>GSHMIRIDATPYPYQFHPRSTALVVIDMQRDFIEEGGFGSALGNDVRPLAAIVPTVAALLQLAREAGMLVVHTRESHLPDLSDCPRSKRLRGNPTLGIGDVGPMGRILVQGEPGNQILPQLAPVEGELVIDKPGKGAFYATDLHAQLQERRITHLLVAGVTTEVCVQTSMREANDRGYECLVIEDA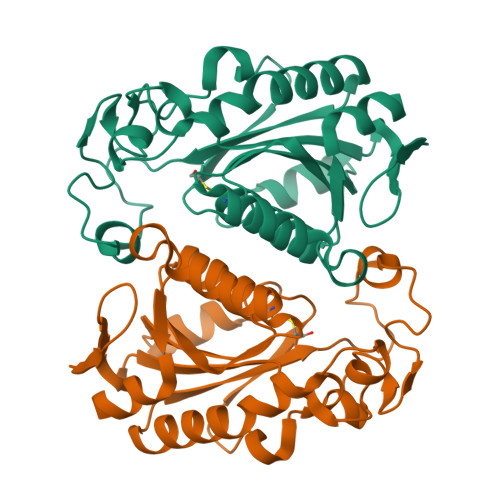CASYFPDFHRITLEMLTAQGGIVGWRTPLAQLQAGVA[8x]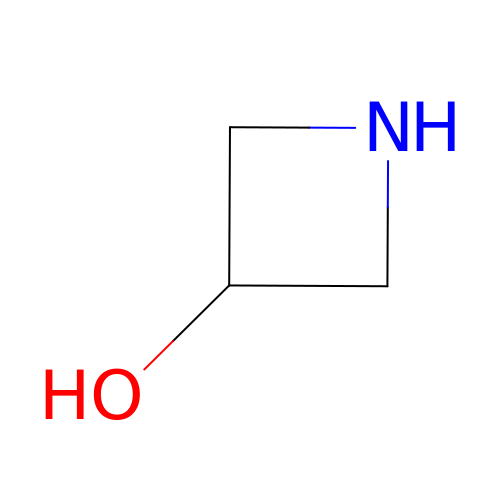azetidin-3-ol | C3 H7 N O | GMWFCJXSQQHBPI-UHFFFAOYSA-N> AKGIAIALLVILVICSLIVT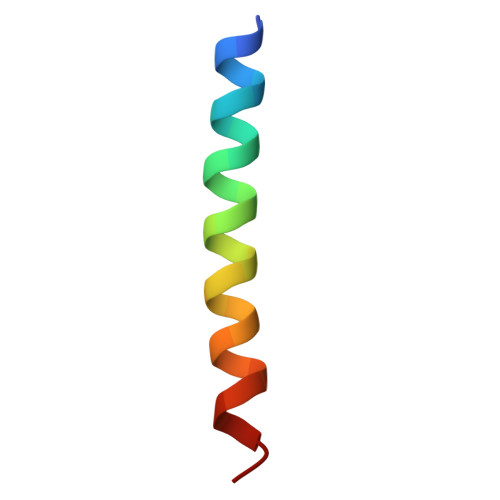SVILLTPA> MEPVKCNLCYECIESDELRA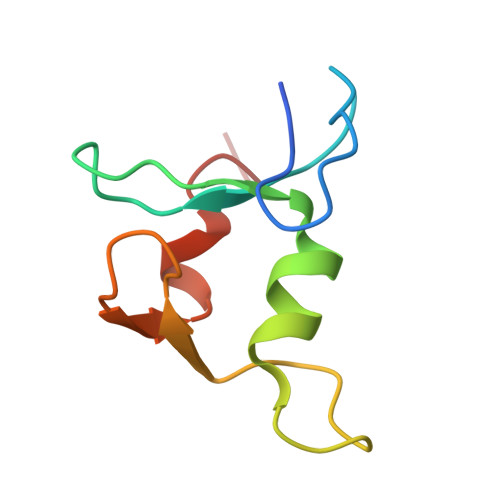NCPFTDCNSINHLTCLASSFLTEECQVLPIEGMCTKCKRVLRWREFLSTVFTT>[6x]MKISDGNWLIQPGLNLI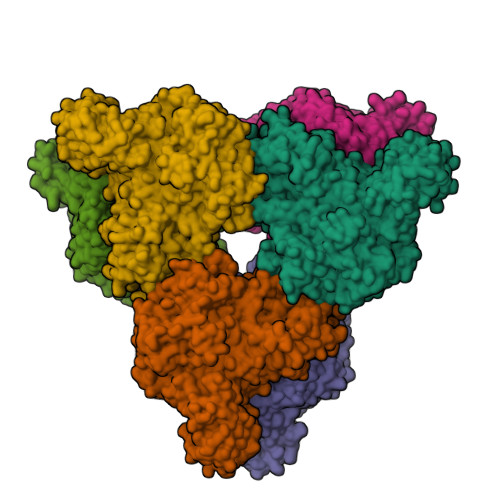HPLQVFEVEQQDNEMVVYAAPRDVRERTWQLDTPLFTLRFFSPQEGIVGVRIEHFQGALNNGPHYPLNILQDVKVTIENTERYAEFKSGNLSARVSKGEFWSLDFLRNGERITGSQVKNNGYVQDTNNQRNYMFERLDLGVGETVYGLGERFTALVRNGQTVETWNRDGGTSTEQAYKNIPFYMTNRGYGVLVNHPQCVSFEVGSEKVSKVQFSVESEYLEYFVIDGPTPKAVLDRYTRFTGRPALPPAWSFGLWLTTSFTTNYDEATVNSFIDGMAERNLPLHVFHFDCFWMKAFQWCDFEWDPLTFPDPEGMIRRLKAKGLKICVWINPYIGQKSPVFKELQEKGYLLKRPDGSLWQWDKWQPGLAIYDFTNPDACKWYADKLKGLVAMGVDCFKTDFGERIPTDVQWFDGSDPQKMHNHYAYIYNELVWNVLKDTVGEEEAVLFARSASVGAQKFPVHWGGDCYANYESMAESLRGGLSIGLSGFGFWSHDIGGFENTAPAHVYKRWCAFGLLSSHSRLHGSKSYRVPWAYDDESCDVVRFFTQLKCRMMPYLYREAARANARGTPMMRAMMMEFPDDPACDYLDRQYMLGDNVMVAPVFTEAGDVQFYLPEGRWTHLWHNDELDGSRWHKQQHGFLSLPVYVRDNTLLALGNNDQRPDYVWHEGTAFHLFNLQDGHEAVCEVPAADGSVIFTLKAARTGNTITVTGAGEAKNWTLCLRNVVKVNGLQDGSQAESEQGLVVKPQGNALTITLHHHHHH Microtubule (MT) nucleation is regulated by the γ-tubulin ring complex (γTuRC), conserved from yeast to humans. In budding yeast, homologues of the grip-containing proteins (GCPs) GCP2 and GCP3 (Spc97p and Spc98p) and two copies of γ–tubulin (Tub4p) form a 300 kDa complex (γTuSC). Spc110p, a distant pericentrin homologue, recruits this complex to the nuclear face of the spindle pole body (SPB), while Spc72p recruits it to the cytoplasmic face. In yeast, the CM1 motif is required for seven identical γTuSCs to helically assemble into a γTuRC at the SPB.

Finally, by local 3D classification we observed that a closed state is populated in our γTuRCWT data. This state had previously not been observed in the γTuRCWT structure as robust symmetry expansion and 3D classification techniques had not yet been developed for cryo-EM when the structure was published. While not identical to the disulfide crosslinked closed state, the differences are minimal, indicating that the conformational changes observed at highest resolution in γTuRCSS are representative of those occurring in the closed WT γTuRCs. The fact that the WT closed state can occur spontaneously and is sampled in our open population suggests that, in the presence of Spc110p, the energy differences between the open and closed states are not large. The observation that a population of γTuRCs in the WT filaments adopts a locally closed conformation indicates a small energetic barrier to a single γTuSC closing, although simultaneous closing of an entire ring is unlikely.

>[2x]MGGEIITLQAGQCGNHVGKFLWSQLAKEHAIGTDGLSQLPDSSTERDDDTKPFFRENSRNKFTPRAIMMDSEPSVIADVENTFRGFFDPRNTWVASDGASAGNSWANGYDIGTRNQDDILNKIDKEIDSTDNFEGFQLLHSVAGGTGSGLGSNLLEALCDRYPKKILTTYSVFPARSSEVVVQSYNTILALRRLIEDSDATVVFDNASLLNISGKVFRNPNIDLQHTNQLISTIISSVTNSIRFPSYMYSSMSSIYSTLIPSPELHFLSPSFTPFTSDYIHDDIAHKGHSSYDVMLDLLDPSNSLVSTAMNNPTYFNVYNTIIGNVEPRQISRAMTKLQQRIKFPSWSSSAMHVNIGRRSPYLPLQPNENEVSGMMLSNMSTVVNVFENACNTFDKVFAKGAFLNNYNVGDLFQSMQNVQDEFAESREVVQSLMEDYVAAEQDSYLDDVLVDDENMVGELEEDLDADGDHKLV;> MELEPTLFGIIEALAPQLLSQSHLQTFVSDVVNLLRSSTKSATQLGPLIDFYKLQSLDSPETTIMWHKIEKFLDALFGIQNTDDMVKYLSVFQSLLPSNYRAKIVQKSSGLNMENLANHEHLLSPVRAPSIYTEASFENMDRFSERRSMVSSPNRYVPSSTYSSVTLRQLSNPYYVNTIPEEDILKYVSYTLLATTSALFPFDHEQIQIPSKIPNFESGLLHLIFEAGLLYQSLGYKVEKFRMLNISPMKKALIIEISEELQNYTAFVNNLVSSGTVVSLKSLYREIYENIIRLRIYCRFTEHLEELSGDTFLIELNIFKSHGDLTIRKIATNLFNSMISLYYEYLMNWLTKGLLRATYGEFFIAENTDTNGTDDDFIYHIPIEFNQERVPAFIPKELAYKIFMIGKSYIFLEKYCKEVQWTNEFSKKYHVLYQSNSYRGISTNFFEIINDQYSEIVNHTNQILNQKFHYRDVVFALKNILLMGKSDFMDALIEKANDILATPSDSLPNYKLTRVLQEAVQLSSLRHLMNSPRNSSVINGLDARVLDLGHGSVGWDVFTLDYILYPPLSLVLNVNRPFGRKEYLRIFNFLWRFKKNNYFYQKEMLKSNDIIRSFKKIRGYNPLIRDIINKLSRISILRTQFQQFNSKMESYYLNCIIEENFKEMTRKLQRTENKSQNQFDLIRLNNGTIELNGILTPKAEVLTKSSSSKPQKHAIEKTLNIDELESVHNTFLTNILSHKLFATNTSEISVGDYSGQPYPTSLVLLLNSVYEFVKVYCNLNDIGYEIFIKMNLNDHEASNGLLGKFNTNLKEIVSQYKNFKDRLYIFRADLKNDGDEELFLLSKSLR;> MEIKEVDDRAELLRYTNNIPLLGKLVNHQPLWSTNPKLKSFSLEKISAPDQRRVQEALVVKDLLNVLIGLEGTYIRYFNDYEPSDPETPIEFKIAKKMDPSFKTFSRRIVRYGKQYMILTRAYEKWSDTSFGMVLQRFAYEIRRFLEDVYLKTLVERLERDFNKVPNFSIRELEQIINETEVNKQMELLYNIYEEIFREIEERRTNQSSQEDFNNFMDSMKNESSLHLRLMVAFDTTVYPVPKGGAILKIFQQKILENLGDRSSVMFLKKLLNNISQDYCTMLYEWLTQGILNDPYQEFMTYDDLEGKTDNIFDTRDRAWDTQYFIRKDVLLRDCDSEEDKNLLFKMLRTGILLKVVRASLQIPTIPSNSSDITIQEINDFADLMEGSNLELYVDKCYSRANEIFLKLFFQGYDLINVLKHLQQIFLGYQSGHNVLKFLTKNMGELTKHYRNDNNANYDKLLQNFELERQSENPNNLMRQLLMIQFDTETLPQVLSHYLQIYPEVPENNSANDDSDPLMHANNFKNMNAILFDELSKERTGAYHGSNLELYTPKSAIYHLKFDINIPYPLNIIISRTCMIKYQIILRYQLVLQYHSRLLDETWMDLNKTPSWKYRGYSHTVKRRIVRATRVLHAKMNHFIKTIMEYFNQNVIDKEVYSLEKCYRNPTLAVAIQNELEGGLTNIMTNRCLSDLIPLQLQIFDIVYKFCKFIKSMRAKLCQLDPVLYEKHKSGMMKTLNEGYRTNNGGQEDVGYQEDAALELIQKLIEYISNASSIFRKCLINFTQELSTEKFDFYDSSSVDAAGIERVLYSIVPPRSASASSQR;> MDEASHLPNGSLKNMEFTPVGFIKSKRNTTQTQVVSPTKVPNANNGDENEGPVKKRQRRSIDDTIDSTRLFSEASQFDDSFPEIKANIPPSPRSGNVDKSRKRNLIDDLKKDVPMSQPLKEQEVREHQMKKERFDRALESKLLGKRHITYANSDISNKELYINEIKSLKHEIKELRKEKNDTLNNYDTLEEETDDLKNRLQALEKELDAKNKIVNSRKVD(2~{S})-~{N}-[5-(5-azanylpyridin-3-yl)-4-ethanoyl-1,3-thiazol-2-yl]piperazine-2-carboxamide | C15 H18 N6 O2 S | 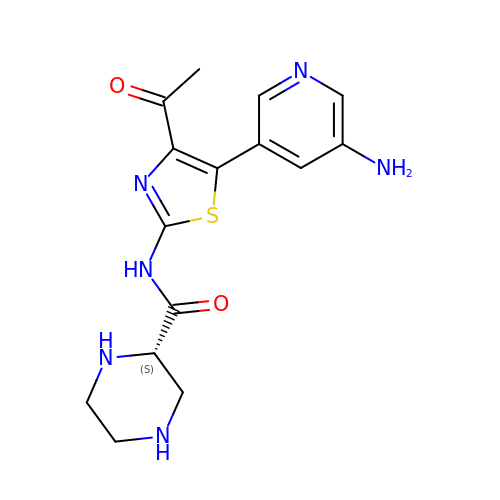CTUFUQNJXFRTNL-NSHDSACASA-N(1~{R},3~{S},5~{Z})-4-methylidene-5-[(~{E})-3-[3-(6-methyl-6-oxidanyl-heptyl)phenyl]non-2-enylidene]cyclohexane-1,3-diol | C30 H46 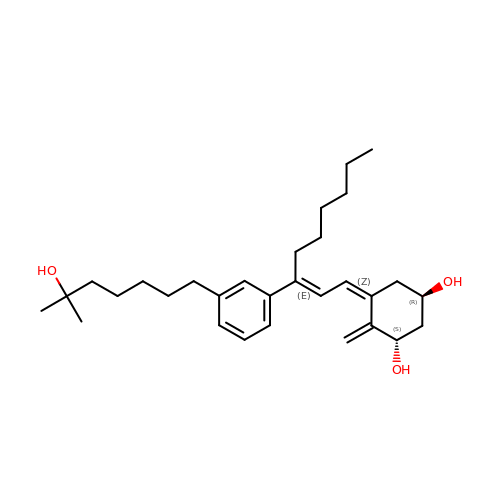O3 | ISCBFPXNVUJFJI-HSDCXWRNSA-N>[4x]MSKIKNPILTGFHPDPSICRVGDDYYIAVSTFEWFPGVRIYHSKDLKNWRLVARPLNRLSQLNMIGNPDSGGVWAPHLSYSDGKFWLIYTDVKVVEGQWKDG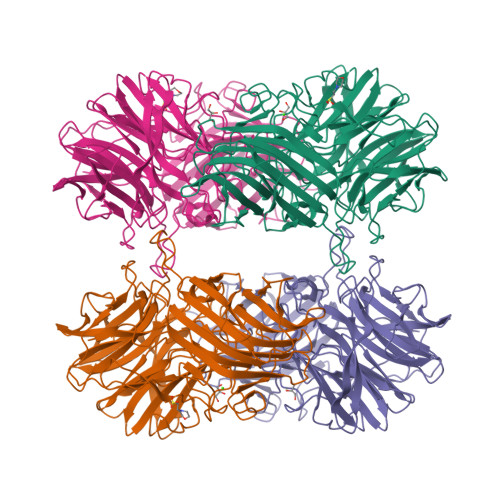HNYLVTCDTIDGAWSDPIYLNSSGFDPSLFHDEDGRKYLVNMYWDHRVDHHPFYGIVLQEYSVEQKKLVGEPKIIFKGTDLRITEGPHLYKINGYYYLLTAEGGTRYNHAATIARSTSLYGPYEVHPDNPLLTSWPYPRNPLQKAGHASIVHTHTDEWFLVHLTGRPLPREGQPLLEHRGYCPLGRETAIQRLEWKDGWPYVVGGNGPSLEIDGPSVEEVSWEKDYDEKDDFDGDTLNHHFQTLRIPLGEDIATLKARPGHLRLYGRESLTSRFTQAFVARRWQHFHFVAETKVSFRPTTFQQSAGLVNYYNTQNWTTLQITWHEEKGRILELMTCDHLVVDQPLRGREIVVPDDIEYVYLRVTVQATTYKYSYSFDGMNWIDLPVTFESYKLSDDYIKSRAAFTGAFVGMHCRDGSGQNNYADFDYFLYKEL> MELQPQFNEFLANIRPTDTQKEDWKSGARTLRERLKNFEPLKEIVVSTFLQGSIRRSTAIRPLGDKRPKVKIVVVTNLDHTRMSPTDAMDLFIPFLEKYYPGKWETQGRSFGITLSYVELDLVITAIPESGAEKSHLEQLYKSESVLTVNSLEEQTDWRLNKSWTPNTGWLSESNSAQVEDAPASEWKAHPLVLPDREKNEWGRTHPLAQIRWTAEKNRLCNGHYINLVRAVKWWRQQNSEDLPKYPKGYPLEHLIGNALDNGTTSMAQGLVQLMDTFLSRWAAIYNQKSKPWLSDHGVAEHDVMARLTAEDFCSFYEGIASAAEIARNALASEEPQESAQLWRQLFGSKFPLPGPQGGD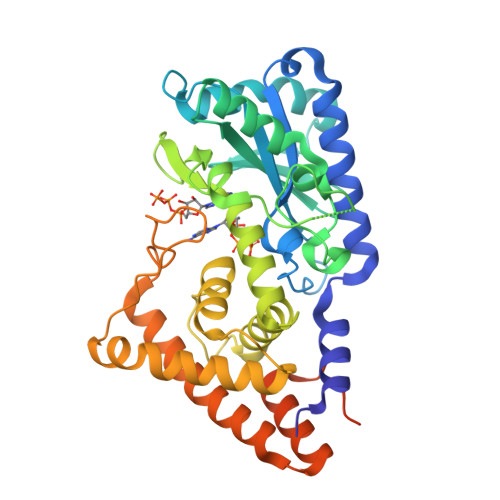RNGGFTTPSKPAEPQKTGRFALEHHHHHH> GTSTQTKAGSLTIVGTGIESIGQMTLQALSYIEAAAKVFYCVIDPATEAFILTKNKNCVDLYQYYDNGKSALNTYTQMSELMVREVRKGLDVVGVFYGHPGVFVNPSHRALAIAKSEGYRARMLPGVSAEDCLFADLCIDPSNPGCLTYEASDFLIRDRPVSIHSHLVLFQVGCVGI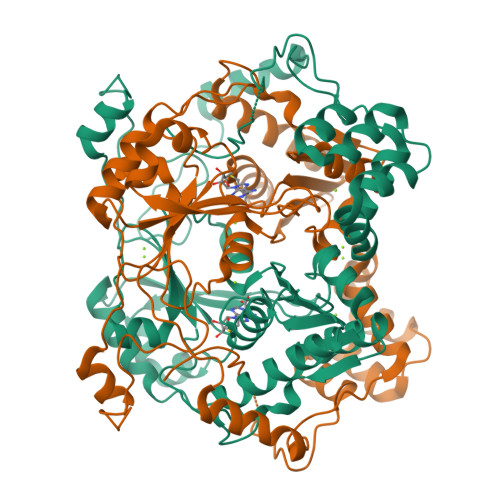ADFNFTGFDNNKFGVLVDRLEQEYGAEHPVVHYIAAMMPHQDPVTDKYTVAQLREPEIAKRVGGVSTFYIPPKARKASNLDIIRRLELLPAGQVPDKKARIYPANQWEPDVPEVEPYRPSDQAAIAQLADHAPPEQYQPLATSKAMSDVMTKLALDPKALADYKADHRAFAQSVPDLTPQERAALELGDSWAIRCAMKNMPSSLLDAARESGEEASQNGFPWVIVVGVIGVIG In previous work we have explored the potential for establishing a bump-&-hole system targeting the bromodomains of the BET (bromo and extra-terminal) protein family. These four human proteins – BRD2, BRD3, BRD4 and BRDT – each contain two tandem bromodomains that bind acetylated lysine residues in histone tails, leading to the recruitment of multi-protein complexes to chromatin. Through this function the BET proteins play a significant role in controlling transcription and regulating gene expression. The phenotypes generated by said inhibitors have been used to investigate the functions of BET proteins and their significance as therapeutic targets. This process has been limited by the pan-selective nature of the BET inhibitors, as they typically target all BET bromodomains with similar potency, hence specific proteins/bromodomains cannot be associated to specific phenotypes. Through structural analysis of the bromodomain we hypothesized that a leucine/valine substitution (L/V) would be a more conservative change than the previous L/A substitution, resulting in a smaller ‘hole’ but still allowing enough space to accommodate a bumped ligand.

We therefore decided to replace the methyl-ester side-group first with an amide, as in I-BET762, which would lock the side-group in place through a hydrogen bond from the amide NH to the ASN140 residue. The replacement of the methyl-ester with an amide group results in a pronounced reduction on WT binding affinities. Co-crystal structures confirm the formation of the expected hydrogen bond to Asn140. As this hydrogen bond locks the bump in an orientation facing the WT leucine residue it exacerbates the steric clash. Methyl, ethyl and allyl bumps, the 9′ methoxy group and the ethyl-amide side-group typically met our criteria.

>SMGKLSEQLKHCNGILKELLSKKHAAYAWPFYKPVDASALGVHDYHDIIKHPMDLSTVKRKMENRDYRDAQEFAADVRLMFSNCYKYNPPDHDVVAMARKLQDVFEFRYAKMPD[2x]>[2x]HMVPMDKTLKEFGADVQWDDYAQLFTLIKDGAYVKVKPGAQTAIVNGQPLALQVPVVMKDNKAWVSDTFINDVFQSGLDQTFQVEKRPHPLNALTADEIKQAVEIVKASADFKPNTRFTEISLLPPDKEAVWAFALENKPVDQPRKADVIMLDGKHIIEAVVDLQNNKLLSWQPIKDAHGMVLLDDFASVQNIINNSEEFAAAVKKRGITDAKKVITTPLTVGYFDGKDGLKQDARLLKVISYLDVGDGNYWAHPIENLVAVVDLEQKKIVKIEEGPVVPVPMTARPFDGRDRVAPAVKP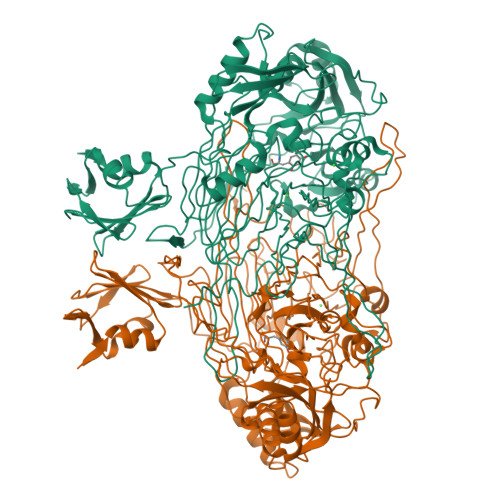MQIIEPEGKNYTITGDMIHWRNWDFHLSMNSRVGPMISTVTYNDNGTKRKVMYEGSLGGMIVPYGDPDIGWYFKAYLNSGDYGMGTLTSPIARGKDAPSNAVLLNETIADYTGVPMEIPRAIAVFERYAGPEYKHQEMGQPNVSTERRELVVRWISTVGNYDYIFDWIFHENGTIGIDAGATGIEAVKGVKAKTMHDETAKDDTRYGTLIDHNIVGTTHQHIYNFRLDLDVDGENNSLVAMDPVVKPNTAGGPRTSTMQVNQYNIGNEQDAAQKFDPGTIRLLSNPNKENRMGNPVSYQIIPYAGGTHPVAKGAQFAPDEWIYHRLSFMDKQLWVTRYHPGERFPEGKYPNRSTHDTGLGQYSKDNESLDNTDAVVWMTTGTTHVARAEEWPIMPTEWVHTLLKPWNFFDETPTLGALKKD>MHHHHHHGHNSNLQDILAANAKWASQMNNIQPTLFPDHNAKGQSPHTLFIGCSDSRYNENCLGVLPGEVFTWKNVANICHSEDLTLKATLEFAIICLKVNKVIICGHTDCGGIKTCLTNQREALPKVNCSHLYKYLDDIDTMYHEESQNLIHLK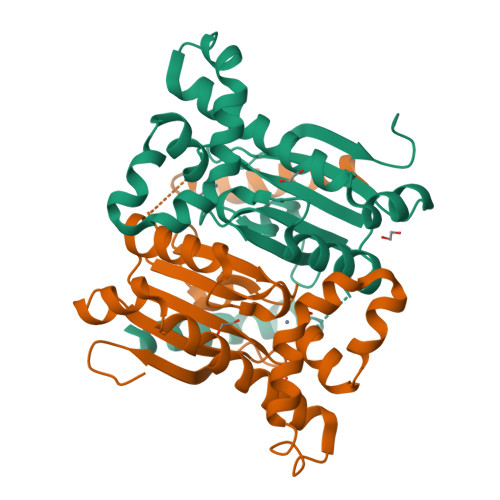TQREKSHYLSHCNVKRQFNRIIENPTVQTAVQNGELQVYGLLYNVEDGLLQTVSTYTKVTPK[2x]>AQYEDGKQYTTLEKPVAGAPQVLEFFSFFCPHCYQFEEVLHISDNVKKKLPEGVKMTKYHVNFMGGDLGKDLTQAWAVAMALGVEDKVTVPLFEGVQKTQTIRSASDIRDVFINAGIKGEEYDAAWNSFVVKSLVAQQEKAAAD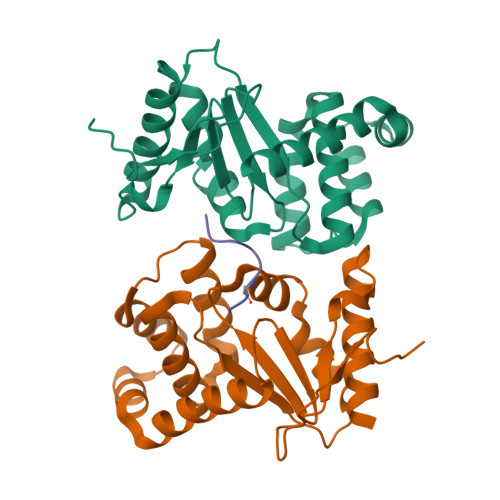VQLRGVPAMFVNGKYQLNPQGMDTSNMDVFVQQYADTVKYLSEEK[4x];>[2x]XPIPFLSQKD3-(PYRIDIN-3-YL)-1H-PYRAZOL-5-AMINE 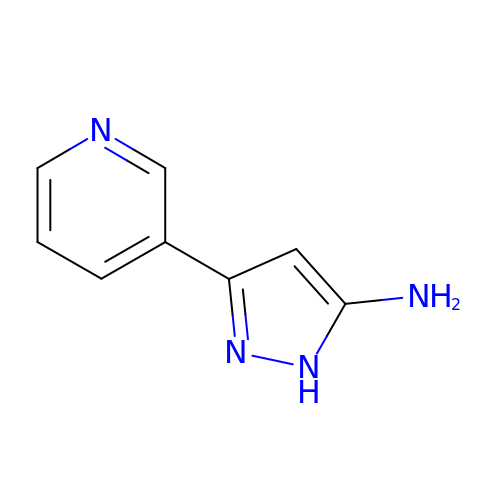| C8 H8 N4 | USKHSGIEOVXVFW-UHFFFAOYSA-N methanesulfonic acid | C H4 O3 S | 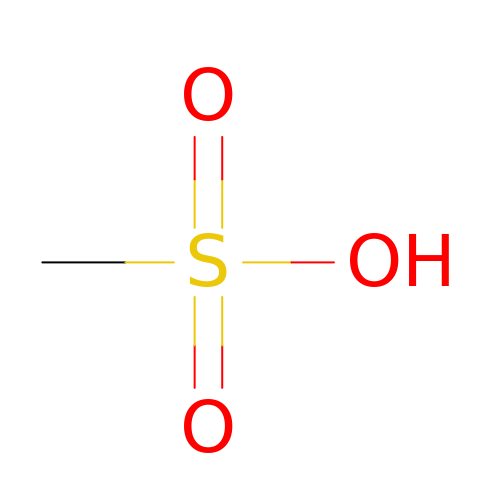AFVFQIVMOAPDHO-UHFFFAOYSA-N>[4x]HHHH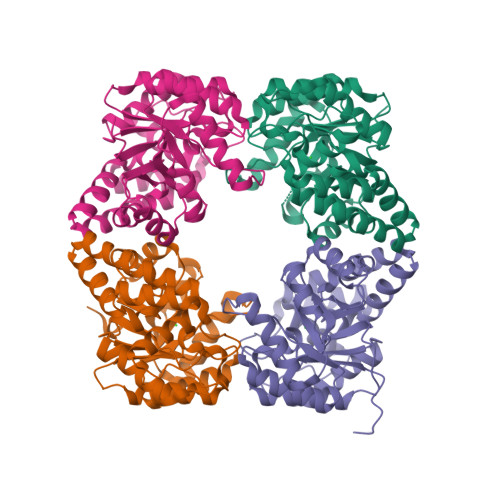HHNKDLKGLYAALLVPFDENGQVNEQGLKQIAQNAIETEELDGLYVNGSSGENFLLNTEQKKQVFKVAKEAVGDKVKLIAQVGSLDLNEAIELGKYATELGYDALSAVTPFYYPFTFEEIRDYYFDIIEATQNNMIIYAIPDLTGVNISIEQFSELFNHEKIVGVKYTAPNFFLLERIRKAFPDKLILSGFDEMLVQATISGVDGAIGSTYNVNGRRARKIFDLARQGQIQEAYQLQHDSNDIIETVLSMGIYPTLKEILRHRGIDAGLPKRPFKPFNEAHRQTLDQLIAKYDL> 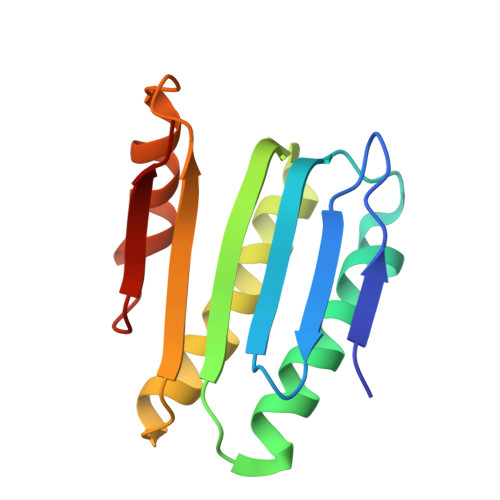SMSDLHIPGTQSTPAIQGDWQAGRLSMQGDSYPENSYELFGQVIDWVERFLADGQRPLELDLRLLYLNTSSIKAMMDILDLLEEAHQGGRPVSLRWHYDRRNERVAELAEEFREDCSFPFAIQAHDE>[8x]MAHHHHHHAALRQPQVAELLAEARRAFREEFGAEPELAVSAPGRVNLIGEHTDYNQGLVLPMALELMTVLVGSPRKDGLVSLLTT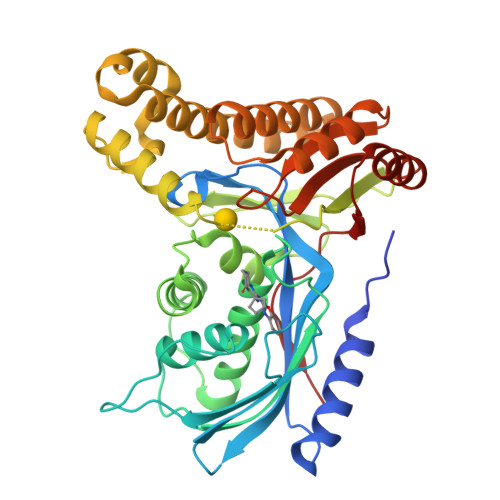SEGADEPQRLQFPLPTAQRSLEPGTPRWANYVKGVIQYYPAAPLPGFSAVVVSSVPLGGGLSSSASLEVATYTFLQQLCPDSGTIAARAQVCQQAEHSFAGMPCGIMDQFISLMGQKGHALLIDCRSLETSLVPLSDPKLAVLITNSNVRHSLASSEYPVRRRQCEEVARALGAASLREVQLEELEAARDLVSKEGFRRARHVVGEIRRTAQAAAALRRGDYRAFGRLMVESHRSLRDDYEVSCPELDQLVEAALAVPGVYGSRMTGGGFGGCTVTLLEASAAPHAMRHIQEHYGGTATFYLSQAADGAKVLCL> MKVGQDKVVTIRYTLQVEGEVLDQGELSYLHGHRNLIPGLEEALEGREEGEAFQAHVPAEKAYGPHDPEGVQVVPLSAFPEDAEVVPGAQFYAQD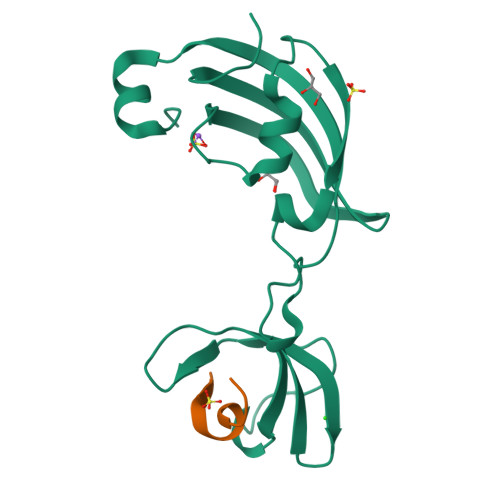MEGNPMPLTVVAVEGEEVTVDFNHPLAGKDLDFQVEVVKVREATPEELLHGHAHPSGHHHHHH;> KMKPFIFGARNKVHIYX> GTTAKQAEAVEDSDINPWTGQRHSERYFKILKARRKLPVNKQRQEFLDLYHNNQILVFVGETGSGKTTQIPQYVLYDELPHQTGKLIACTQPRRVAAMSVAQRVADELDVKLGEEVGYSIRFENKTSSKTLLKYMTDGQLLREAMHDRDMSRYSCIILDEAHERTLATDILMALLKQLSERRKDLKIIVMSATLDAQKFQSYFFNAPLLAVPGRTHPVEIFYTPEAERDYVEAAIRTVLQIHACEPEGDILLFLTGEEEIEDACRRISLEVDEMIRESDAGPMSVYPLYGT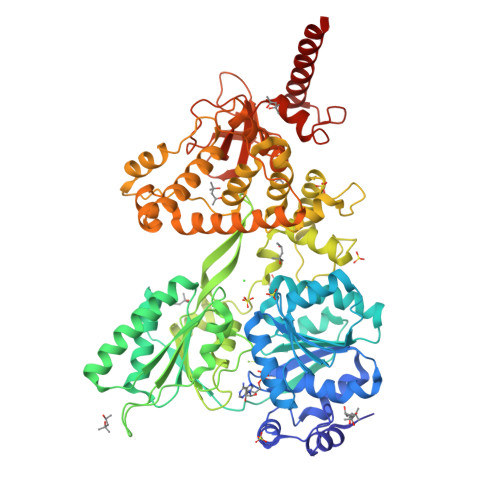LPPHQQQRIFEKAPQPFRPGGRPGRKCIVATNIAETGLTIDGIVYVVDPGFSKQKIYNPRTRVESLLVSPISKASAQQRAGRAGRTRPGKCFRLYTEEAFKKELIEQTYPEILRSNLSNTVLELKKLGVEDLVHFDLMDPPAPETMMRALEELNYLACLDDDGELTPLGNLASEFPLDPALAVMLISSPEFYCSNEILSITSLLSVPQIWVRPANARKRADEMKAQFAHPDGDHLTLLNAYHAYKGAEARGEDMKKWCHEHFLSYRHLSSADNVRAQLKKIMETHGIELVSTPFHDKNYYTNIRRALLAGFFMQVAMRESSNSKVYKTVKDEQLVLIHPSTTVTTPYEWVVYNEFVLTTKQYVRTVTNIRPEWLLEIAPVYYDLSTFQKGEIKNALTRVAEKIRRQQAMKASKA>[2x]QSYTLKDSLSGKDFLDAFSFFADRDPTNGFVHYVSREVAEGEGLVKVTSSGSVYLGVDHTNTLSLTDIGRKSVRLESTDKIDHGLVIADIKHMPGSICGAWPAFWTVGDTWPDDGEIDIIEGVNTQSQNTMVLHTKGNCEITS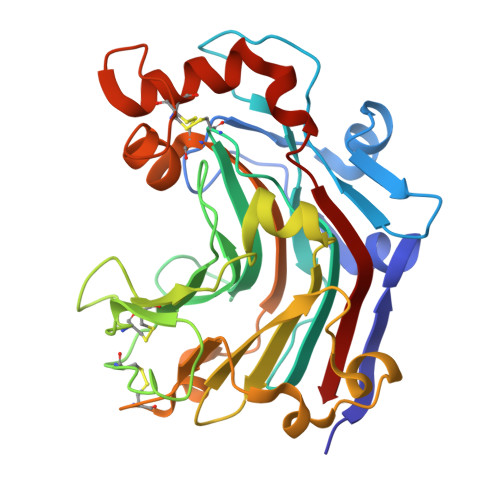DDDQTGTTTSNQCSLDAGPAGCVVQGTPGSYGSSFNEQGGGVYAMQWTDEFIKLWFFPRSAIPKSIESDSPDVSEFGTPMGNFKGTCDIGKEFKPQKLVFDTTFCGDWAGSVYGQSDSCPLTKEDSLASCIDFVATKPEEFKEAYWEINYLKTYT> MPPGVDCPMEFWTKEENQSVVVDFLLPTGVYLNFPVSRNANLSTIKQLLWHRAQYEPLFHMLSGPEAYVFTCINQTAEQQELEDEQRRLCDVQPFLPVLRLVAREGDRVKKLINSQISLLIGKGLHEFDSLCDPEVNDFRAKMCQFCEEAAARRQQLGWEAWLQYSFPLQLEPSAQTWGPGTLRLPNRALLVNVKFEGSEESFTFQVSTKDVPLALMACALRKKATVFRQPLVEQPEDYTLQVNGRHEYLYGSYPLCQFQYICSCLHSGLTPHLTMVHSSSILAMRDEQSNPAPQVQKPRAKPPPIPAKKPSSVSLWSLEQPFRIELIQGSKVNADERMKLVVQAGLFHGNEMLCKTVSSSEVSVCSEPVWKQRLEFDINICDLPRMARLCFALYAVIEKAKKARSTKKKSKKADCPIAWANLMLFDYKDQLKTGERCLYMWPSVPDEKGELLNPTGTVRSNPNTDSAAALLICLPEVAPHPVYYPALEKILELGRHSECVHVTEEEQLQLREILERRGSGELYEHEKDLVWKLRHEVQEHFPEALARLLLVTKWNKHEDVAQMLYLLCSWPELPVLSALELLDF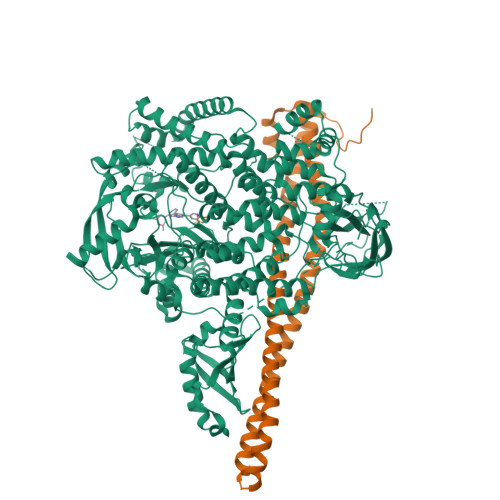SFPDCHVGSFAIKSLRKLTDDELFQYLLQLVQVLKYESYLDCELTKFLLDRALANRKIGHFLFWHLRSEMHVPSVALRFGLILEAYCRGSTHHMKVLMKQGEALSKLKALNDFVKLSSQKTPKPQTKELMHLCMRQEAYLEALSHLQSPLDPSTLLAEVCVEQCTFMDSKMKPLWIMYSNEEAGSGGSVGIIFKNGDDLRQDMLTLQMIQLMDVLWKQEGLDLRMTPYGCLPTGDRTGLIEVVLRSDTIANIQLNKSNMAATAAFNKDALLNWLKSKNPGEALDRAIEEFTLSCAGYCVATYVLGIGDRHSDNIMIRESGQLFHIDFGHFLGNFKTKFGINRERVPFILTYDFVHVIQQGKTNNSEKFERFRGYCERAYTILRRHGLLFLHLFALMRAAGLPELSCSKDIQYLKDSLALGKTEEEALKHFRVKFNEALRESWKTKVNWLAHNVSKDNRQ;> YQQDQVVKEDNIEAVGKKLHEYNTQFQEKSREYDRLYEDYTRTSQEIQMKRTAIEAFNETIKIFEEQCQTQERYSKEYIEKFKREGNETEIQRIMHNYEKLKSRISEIVDSRRRLEEDLKKQAAEYREIDKRMNSIKPDLIQLRKTRDQYLMWLTQKGVRQKKLNEWLG> MASWSHPQEKGALEVLFQ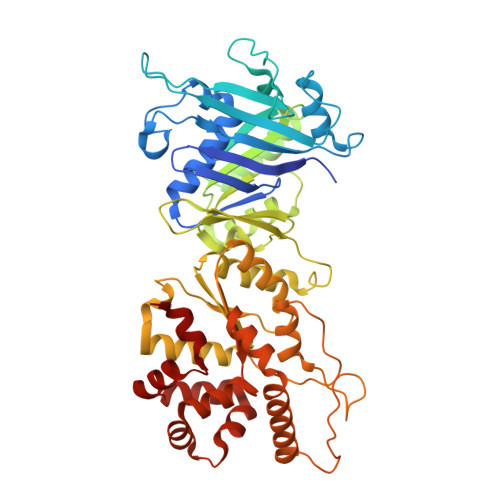GPMKFSNITIKNFRNFEKVNINLDNKNVIFGMNDIGKTNFLYALRFLLDKEIRKFGFNKSDYHKHDTSKKIEIILTLDLSNYEKDEDTKKLISVVKGARTSANADVFYIALESKYDDKELYGNIILKWGSELDNLIDIPGRGNINALDNVFKVIYINPLVDLDKLFAQNKKYIFEESQGNESDEGILNNIKSLTDQVNQQIGEMTIIKGFQQEITSEYRSLKKEEVSIELKSEMAIKGFFSDIIPYIKKDGDSNYYPTSGDGRRKMLSYSIYNYLAKKKYEDKIVIYLIEEPEISLHRSMQIALSKQLFEQSTYKYFFLSTHSPELLYEMDNTRLIRVHSTEKVVCSSHMYNVEEAYGSVKKKLNKALSSALFAERVLLIEGPSEKILFEKVLDEVEPEYELNGGFLLEVGGTYFNHYVCTLNDLGITHIIKTDNDLKSKKGKKGVYELLGLNRCLNLLGRENLDEITIDIPEDIKGKKKKERLNERKKEIFKQYKNEVGEFLGERIYLSEIDLENDLYSAIGESMKRIFENEDPVHYLQKSKLFNMVELVNNLSTKDCFDVFEHEKFACLKELVGSDRG>[3x]MKTRLEQVLERYLNGREVAVWGVPTRRLLRALKPFKFHTADRVDPQYHYVVAVTDDDLTDFLSD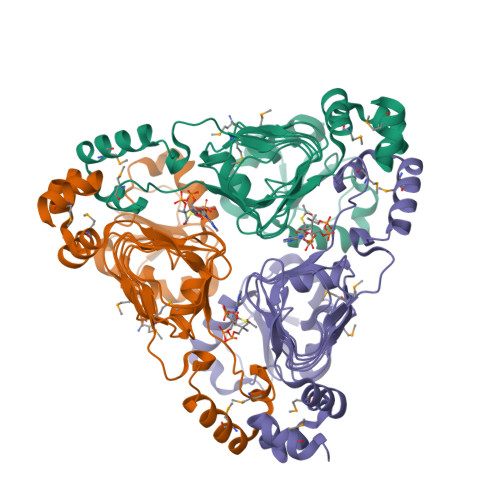EQSKSFQYANDYLTFDDEGGELPFERMCFNVPVGRQTYFGDGVVGACENGYIKSIGQFTSINGTAEIHANHQLNMTFVSDDIQNFFNEESMAVFQEKLRKDPKHPYAYSKEPMTIGSDVYIGAHAFINASTVTSIGDGAIIGSGAVVLENVPPFAVVVGVPARIKRYRFSKEMIETLLRVKWWDWSIEEINENVDALISPELFMKKYGSL> MQPINTSNPDNTASYVKDEVEITSSTIALSEIVSVVNTSDGRLEVFGVGTDKAVWHNRQMAPHTGSPWSGWSSLKGQVTSKPVVYINTDGRLEVFARGTDNALWHIWQTATNAGWSNWQSLGGVITSNPAIYANTDGRLEVFARGADNALWHISQTTAHSGPWSSWASL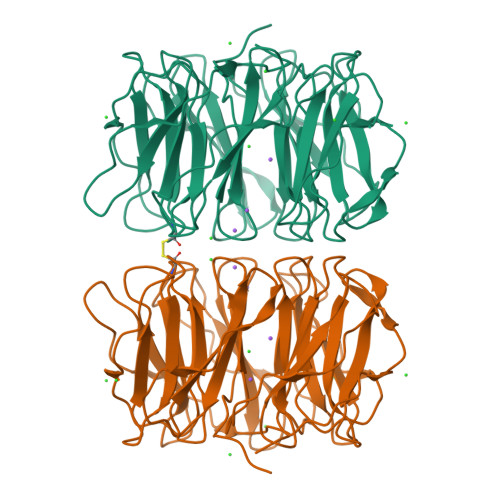NGVITSNPTVHINSDGRLEVFARGTDNALWHIWQTAPDSNLWSSWESLNGIITSDPVVIDTADGRLEVFARGADNALWHIWQTISHSGPWSGWQSLNGVITSAPAVAKNCDNRLEAFARGTDNALWHTWQTVSHSGPWSSWQSLNGVITSAPTAVRDADGRLEVFARGTDNALWLTWQTASSWSPWISLGGVLIDASAIK>[4x]MYYFIPSWSGSGKRVWHRDIIPWYRSMQRLEFDDTIHQIRIFHSENLPVKLLLQAYMPHARYFLHRQDIFETEYYSVFDEIQAVESNDMQVLQIKDLEWEDDCEFIYTPFLIIVRRQGQLYAHVEFGVEGFISFIKFFKDDQLEKLNIFDDRGFVSSIVYYEDGQEVCQDYLNPNGDWRIREYLKFENSHVVVNPVFSRDFDKLEYECMPDLILEKLGYYISHNVEEDSRFVVAAQPFTNQGVLDLLPQHSHSILSFF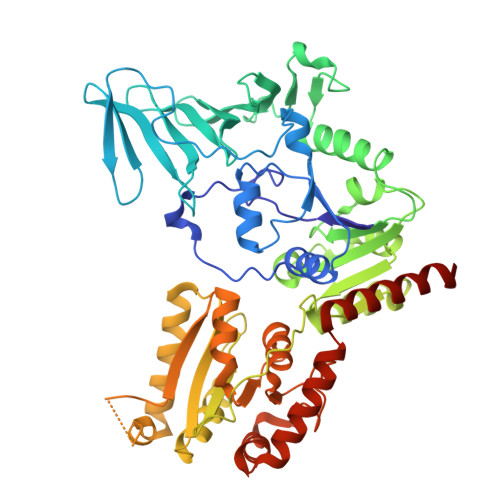HERNQASNIENLKADLEYADLVLTDRMDFKETLQNYFPLQAEKIHYLSPFDTRLQLGKSQQRHESKIFYQIDLSELLNDYAIFKVLFYVAQHPDTELVIGVYNAWQEGIKQVENKVEELISDYLDLKDFIKKSFKNNQAENPLPENQELEYRFRIRNITDELSLIQELDDTRLIIDLSQQPNLYTQIAGISAGIPQINLVASDYVTHLQNGYILDSISQLAVAADYYLQGLKNWNQALIYSIEKIKLNTGHQVIKRWEKWLKEAIDEKVDKLVPR>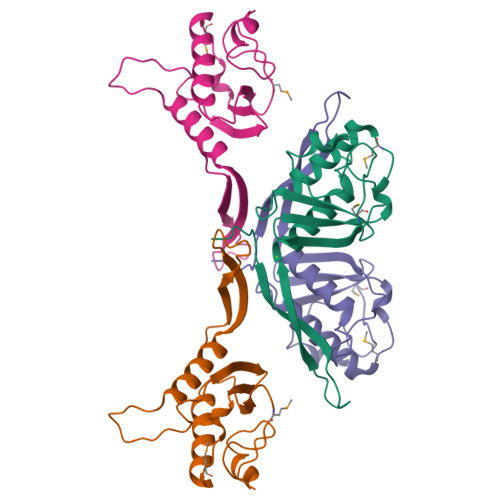[4x]SNADKLAANNNERVKTIANDLIGDIDLSLYFDGTKDEQNPKIEQQEILVDGDEILGQYLIQALIQGPSQKGSLAPILPKDTKLLSFDIKDDIAIINLSKEAIVNMSATKEQATLEGIIATITQIPSINKINILVDNQMVDSLGGNFDISKPFGKEDIPNLKINN> MAYVLDTNVAIHLRDGDPEVTTRVTALNGAILL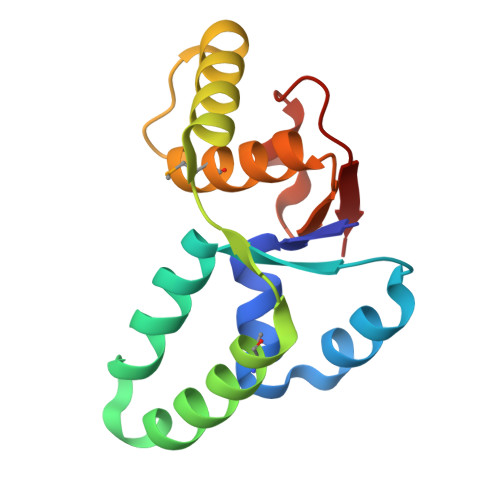SIISRVELEGGVYREAAQAGLRRSRLDVMLKVLPVLDFDGAAADEYRRIVESAGYSRRKVVDRMIAAQALAHRATFVTFNADDFRDIPGLSLLAW>[2x]MSLVLNDLLICCRQLEHDRATERKKEVEKFKRLIRDPETIKHLDRHSDSKQGKYLNWDAVFRFLQKYIQKETECLRIAKPNVSASTQASRQKKMQEISSLVKYFIKCANRRAPRLKCQELLNYIMDTVKDSSNGAIYGADCSNILLKDILSVRKYWCEISQQQWLELFSVYFRLYLKPSQDVHRVLVARIIHAVTKGCCSQTDGLNSKFLDFFSKAIQCARQEKSSSGLNHILAALTIFLKTLAVNFRIRVCELGDEILPTLLYIWTQHRLNDSLKEVIIELFQLQIYIHHPKGAKTQEKGAYESTKWRSILYNLYDLLVNEISHIGSRGKYSSGFRNIAVKENLIELMADICHQVFNEDTRSLEISQSYTTTQRESSDYSVPCKRKKIELGWEVIKDHLQKSQNDFDLVPWLQIATQLISKYPASLPNCELSPLLMILSQLLPQQRHGERTPYVLRCLTEVALCQDKRSNLESSQKSDLLKLWNKIWCITFRGISSEQIQAENFGLLGAIIQGSLVEVDREFWKLFTGSACRPSCPAVCCLTLALTTSIVPGTVKMGIEQNMCEVNRSFSLKESIMKWLLFYQLEGDLENSTEVPPILHSNFPHLVLEKILVSLTMKNCKAAMNFFQSVPECEHHQKDKEELSFSEVEELFLQTTFDKMDFLTIVRECGIEKHQSSIGFSVHQNLKESLDRCLLGLSEQLLNNYSSEITNSETLVRCSRLLVGVLGCYCYMGVIAEEEAYKSELFQKAKSLMQCAGESITLFKNKTNEEFRIGSLRNMMQLCTRCLSNCTKKSPNKIASGFFLRLLTSKLMNDIADICKSLASFIKKPFDRGEVESMEDDTNGNLMEVEDQSSMNLFNDYPDSSVSDANEPGESQSTIGAINPLAEEYLSKQDLLFLDMLKFLCLCVTTAQTNTVSFRAADIRRKLLMLIDSSTLEPTKSLHLHMYLMLLKELPGEEYPLPMEDVLELLKPLSNVCSLYRRDQDVCKTILNHVLHVVKNLGQSNMDSENTRDAQGQFLTVIGAFWHLTKERKYIFSVRMALVNCLKTLLEADPYSKWAILNVMGKDFPVNEVFTQFLADNHHQVRMLAAESINRLFQDTKGDSSRLLKALPLKLQQTAFENAYLKAQEGMREMSHSAENPETLDEIYNRKSVLLTLIAVVLSCSPICEKQALFALCKSVKENGLEPHLVKKVLEKVSETFGYRRLEDFMASHLDYLVLEWLNLQDTEYNLSSFPFILLNYTNIEDFYRSCYKVLIPHLVIRSHFDEVKSIANQIQEDWKSLLTDCFPKILVNILPYFAYEGTRDSGMAQQRETATKVYDMLKSENLLGKQIDHLFISNLPEIVVELLMTLHEPANSSASQSTDLCDFSGDLDPAPNPPHFPSHVIKATFAYISNCHKTKLKSILEILSKSPDSYQKILLAICEQAAETNNVYKKHRILKIYHLFVSLLLKDIKSGLGGAWAFVLRDVIYTLIHYINQRPSCIMDVSLRSFSLCCDLLSQVCQTAVTYCKDALENHLHVIVGTLIPLVYEQVEVQKQVLDLLKYLVIDNKDNENLYITIKLLDPFPDHVVFKDLRITQQKIKYSRGPFSLLEEINHFLSVSVYDALPLTRLEGLKDLRRQLELHKDQMVDIMRASQDNPQDGIMVKLVVNLLQLSKMAINHTGEKEVLEAVGSCLGEVGPIDFSTIAIQHSKDASYTKALKLFEDKELQWTFIMLTYLNNTLVEDCVKVRSAAVTCLKNILATKTGHSFWEIYKMTTDPMLAYLQPFRTSRKKFLEVPRFDKENPFEGLDDINLWIPLSENHDIWIKTLTCAFLDSGGTKCEILQLLKPMCEVKTDFCQTVLPYLIHD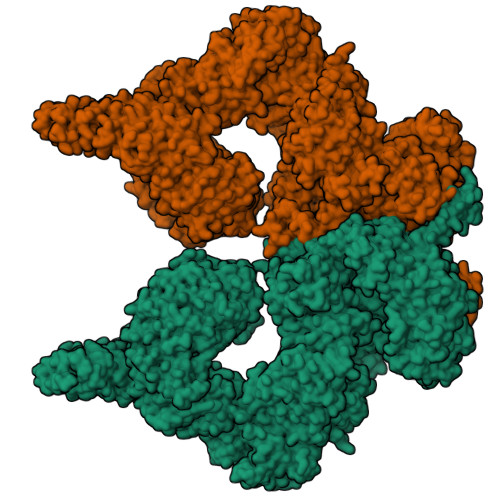ILLQDTNESWRNLLSTHVQGFFTSCLRHFSQTSRSTTPANLDSESEHFFRCCLDKKSQRTMLAVVDYMRRQKRPSSGTIFNDAFWLDLNYLEVAKVAQSCAAHFTALLYAEIYADKKSMDDQEKRSLAFEEGSQSTTISSLSEKSKEETGISLQDLLLEIYRSIGEPDSLYGCGGGKMLQPITRLRTYEHEAMWGKALVTYDLETAIPSSTRQAGIIQALQNLGLCHILSVYLKGLDYENKDWCPELEELHYQAAWRNMQWDHCTSVSKEVEGTSYHESLYNALQSLRDREFSTFYESLKYARVKEVEEMCKRSLESVYSLYPTLSRLQAIGELESIGELFSRSVTHRQLSEVYIKWQKHSQLLKDSDFSFQEPIMALRTVILEILMEKEMDNSQRECIKDILTKHLVELSILARTFKNTQLPERAIFQIKQYNSVSCGVSEWQLEEAQVFWAKKEQSLALSILKQMIKKLDASCAANNPSLKLTYTECLRVCGNWLAETCLENPAVIMQTYLEKAVEVAGNYDGESSDELRNGKMKAFLSLARFSDTQYQRIENYMKSSEFENKQALLKRAKEEVGLLREHKIQTNRYTVKVQRELELDELALRALKEDRKRFLCKAVENYINCLLSGEEHDMWVFRLCSLWLENSGVSEVNGMMKRDGMKIPTYKFLPLMYQLAARMGTKMMGGLGFHEVLNNLISRISMDHPHHTLFIILALANANRDEFLTKPEVARRSRITKNVPKQSSQLDEDRTEAANRIICTIRSRRPQMVRSVEALCDAYIILANLDATQWKTQRKGINIPADQPITKLKNLEDVVVPTMEIKVDHTGEYGNLVTIQSFKAEFRLAGGVNLPKIIDCVGSDGKERRQLVKGRDDLRQDAVMQQVFQMCNTLLQRNTETRKRKLTICTYKVVPLSQRSGVLEWCTGTVPIGEFLVNNEDGAHKRYRPNDFSAFQCQKKMMEVQKKSFEEKYEVFMDVCQNFQPVFRYFCMEKFLDPAIWFEKRLAYTRSVATSSIVGYILGLGDRHVQNILINEQSAELVHIDLGVAFEQGKILPTPETVPFRLTRDIVDGMGITGVEGVFRRCCEKTMEVMRNSQETLLTIVEVLLYDPLFDWTMNPLKALYLQQRPEDETELHPTLNADDQECKRNLSDIDQSFNKVAERVLMRLQEKLKGVEEGTVLSVGGQVNLLIQQAIDPKNLSRLFPGWKAWV>[3x]ADKRIRSDSSAAAVQAMKNAAVDTIDPPSHAGLEKKAEPFWHDNIRSKALDSWTPADLLAAVELANNQLYITVLRKD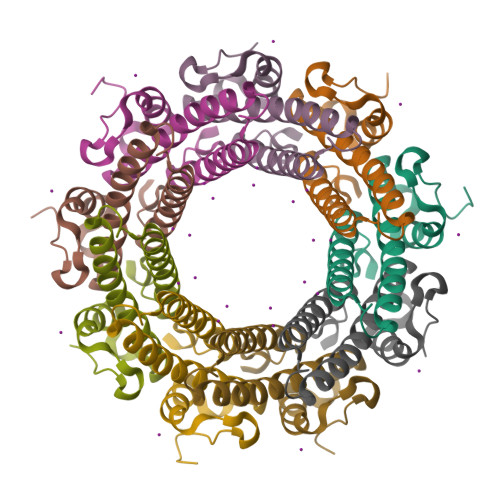LRKEERIRGEERDEGLIKDLRKQIVELQRTILAQRRDLQIHSHATNGESRDQKKRNQNDRDARNTKNEHQDQDDNLIAFPKHG Y-family polymerases are able to bypass a variety of DNA lesions that impede high-fidelity replicative DNA polymerases. 7,8-dihydro-8-oxoguanine (oxoG) is the major known product of oxidation of DNA by reactive oxygen species induced by either ionizing radiation, photochemical mechanisms, or normal cellular metabolic activity. Our kinetic primer extension studies demonstrate that the bypass polymerase Dpo4 preferentially inserts C opposite oxoG, and also preferentially extends from the oxoG•C base pair, thus achieving error-free bypass of this lesion. The Dpo4 polymerase embraces the 19-mer template/13-mer primer DNA by its four domains: palm (residues 1–10 and 78–166), finger (residues 11–77), thumb (residues 167–233), and little-finger (residues 244–341).

We have determined the 1.95-Å crystal structure of the Dpo4 insertion ternary complex with oxoG-modified, 19-mer template/dideoxy-terminated 13-mer primer, and dCTP positioned opposite oxoG. The finger domain, which is on top of the C7•G13 base pair in the active site of the preinsertion binary complex, is now positioned over the replicating oxoG(anti)•dCTP base pair in the active site of the insertion ternary complex. The side chains of the hydrophobic residues V32 and A42 and the backbone of G58 are packed against the purine ring of oxoG, and the hydrophobic residues A44, A57, and Y12 are packed against the pyrimidine and sugar rings of incoming dCTP. The oxygen atoms of the relocated phosphate group form two hydrogen bonds with the guanidine group of Arg331, one hydrogen bond with the guanidine group of Arg332, and two hydrogen bonds with the hydroxyl group of Ser34. The carbonyl oxygen at C8 forms a water-mediated hydrogen bond with the side chain of Arg332, thus helping to lock the oxoG residue in the anti conformation. By contrast, the phosphate group of unmodified G forms only two hydrogen bonds with the guanidine group of Arg332; thus oxoG(anti) forms four more hydrogen bonds with Dpo4 than unmodified G does. We find one Ca2+ ion coordinated by the catalytic triad, the second chelated by the phosphate groups of the incoming dCTP, with the third ion coordinated by the loop of the thumb domain (residues 181 and 186), adjacent to the tip of helix H.

>GSHMGGGGGIVLFVDFDYFYAQVEEVLNPSLKGKPVVVCVFSGRFEDSGAVATANYEARKFGVKAGIPIVEAKKILPNAVYLPMRKEVYQQVSSRIMNLLREYSEKIEIASIDEAYLDISDKVRDYREAYNLGLEIKNKILEKEKITVTVGISKNKVFAKIAADMAKPNGIKVIDDEEVKRLIRELDIADVPGIGNITAEKLKKLGINKLVDTLSIEFDKLKGMIGEAKAKYLISLARDEYNEPIRTRVRKSIGRIVTMKRNSRNLEEIKPYLFRAIEESYYKLDKRIPKAIHVVAVTEDLDIVSRGRTFPHGISKETAYSESVKLLQKILEEDERKIRRIGVRFSKFIEAIGLDKFFDT[2x]> PIFLNVLEAIEPGVVCAGHDNNQPDSFAALLSSLNELGERQLVHVVKWAKALPGFRNLHVDDQMAVIQYSWMGLMVFAMGWRSVTNVNSRMLYFAPDLVFNEYRMHKSRMYSQCVRMRHLSQEFGWLQ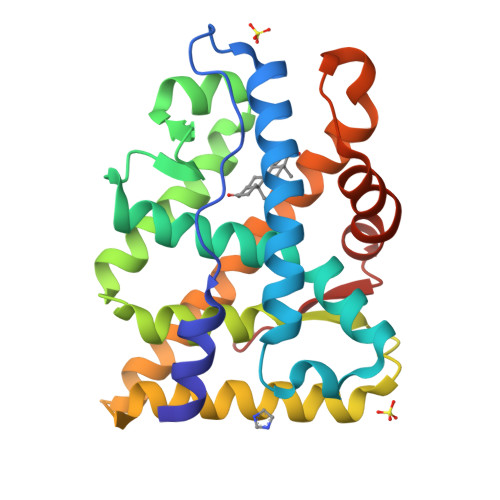ITPQEFLCMKALLLFSIIPVDGLKNQKFFDELRMNYIKELDRIIACKRKNPTSCSRRFYQLTKLLDSVQPIARELHQFTFDLLIKSHMVSVDFPEMMAEIISVQVPKILSGKVKPIYFHTQ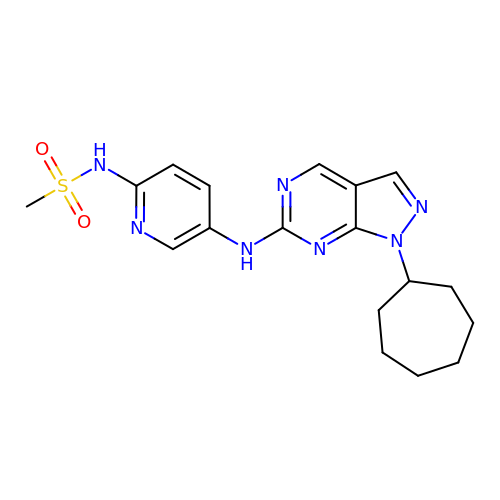N-{5-[(1-cycloheptyl-1H-pyrazolo[3,4-d]pyrimidin-6-yl)amino]pyridin-2-yl}methanesulfonamide | C18 H23 N7 O2 S | PARUULGUCQEWNM-UHFFFAOYSA-N>[2x]SNAMPFLPDPGEPSPLKVVIAGAGYVGTCLAVTLAGRGAEVVAVDSDPGTVADLRAGRCRLPEPGLAGAVRDLAATGRLTASTSYDPVGA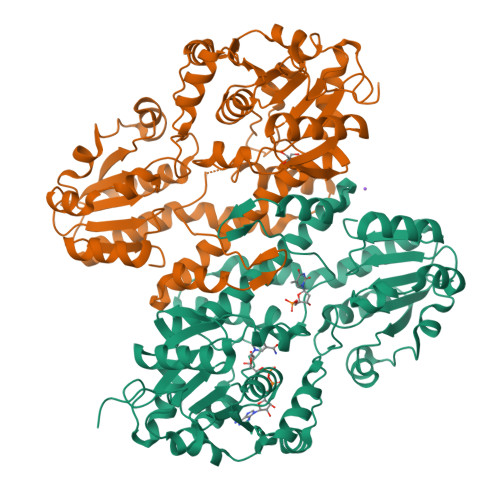ADVVIVTVGTPTDAGHEMVTDQLVAACEQIAPRLRAGQLVILKSTVSPGTTRTLVAPLLESGGLVHERDFGLAFCPERLAEGVALAQVRTLPVVVGGCGPRSAAAAERFWRSALGVDVRQVPSAESAEVVKLATNWWIDANVAIANELARYCAVLGVDVLDVIGAANTLPKGSSMVNLLLPGVGVGGSCLTKDPWMAWRDGRDRGVSLRTVETARAVNDDMPRHTAAVIADELVKLGRDRNDTTIAVLGAAFKNDTGDVRNTPVRGVVAALRDSGFRVRIFDPLADPAEIVARFGTAPAASLDEAVSGAGCLAFLAGHRQFHELDFGALAERVDEPCLVFDGRMHLPPARIRELHRFGFAYRGIGR> AVSLDRTRAVFDGSEKSMTLDISNDNKQLPYLAQAWIENENQEKIITGPVIATPPVQRLDPGAKSMVRLSTTPDISKLPQDRESLF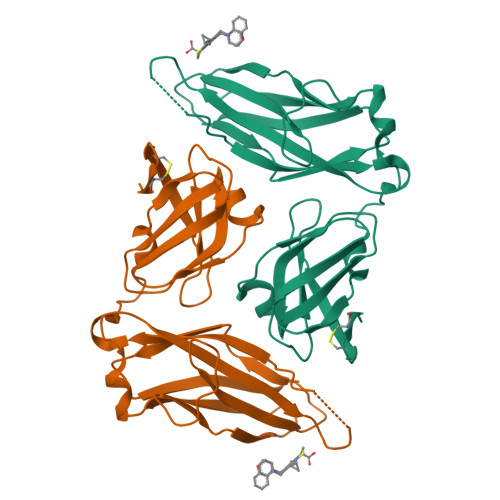YFNLREIPPRSEKANVLQIALQTKIKLFYRPAAIKTRPNEVWQDQLILNKVSGGYRIENPTPYYVTVIGLGGSEKQAEEGEFETVMLSPRSEQTVKSANYNTPYLSYINDYGGRPVLSFICNGSRCSVKKEK> MNVVRYTPWPGQAALQ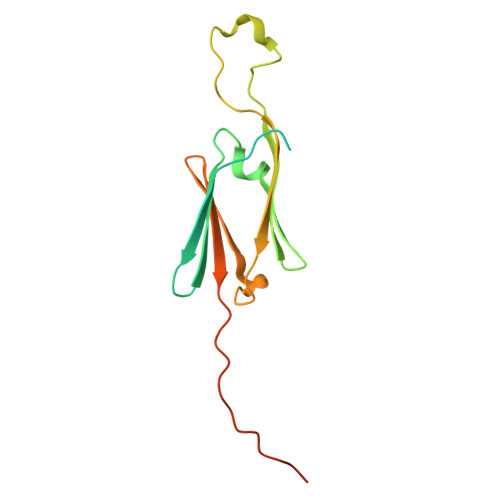NEIKQVFDRFFEHNGDTDESAVVTAQWVPRVDIKEEPNQFVLYADLPGIDPADIEVQMDKGILSIKGERKTESSSQTEHFSRIERRYGSFHRRFALPDSADADGITASGSHGVLSIFIPKRAATTPRRIQVGNAVSNDVALQSM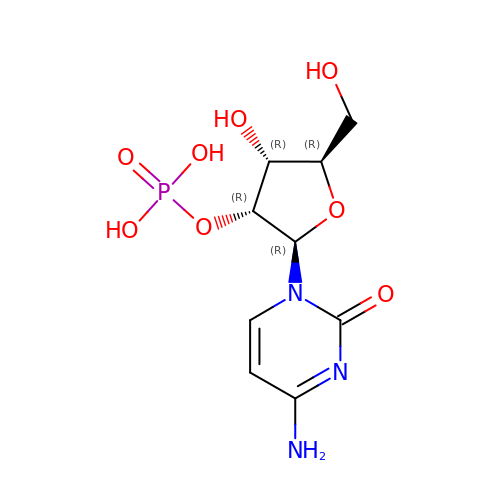CYTIDINE-2'-MONOPHOSPHATE | C9 H14 N3 O8 P | YQUAKORMLHPSLZ-XVFCMESISA-N> MVPSSPAVEKQVPVEPGPDPELRSWRHLVCYLCFYGFMAQIRPGESFITPYLLGPDKNFTREQVTNEITPVLSYSYLAVLVPVFLLTDYLRYTPVLLLQGLSFVSVWLLLLLGHSVAHMQLMELFYSVTMAARIAYSSYIFSLVRPARYQRVAGYSRAAVLLGVFTSSVLGQLLVTVGRVSFSTLNYISLAFLTFSVVLALFLKRPKRSLFFNRDDRGRCETSASELERMNPGPGGKLGHALRVACGDSVLARMLRELGDSLRRPQLRLWSLWWVFNSAGYYLVVYYVHILWNEVDPTTNSARVYNGAADAASTLLGAITSFAAGFVKIRWARWSKLLIAGVTATQAGLVFLLAHTRHPSSIWLCYAAFVLFRGSYQFLVPIATFQIASSLSKELCALVFGVNTFFATIVKTIITFIVSDVRGLG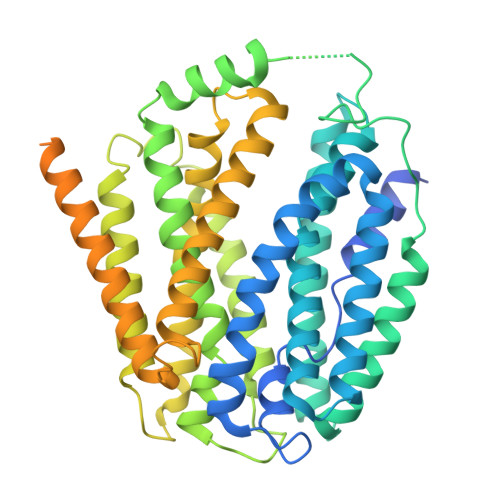LPVRKQFQLYSVYFLILSIIYFLGAMLDGLRHCQRGHHPRQPPAQGLRSAAEEKAAQALSVQDKGLGGLQPAQSPPLSPEDSLGAVGPASLEQRQSDPYLAQAPAPQAAEFLSPVTTPSPCTLCSAQASGPEAADETCPQLAVHPPGVSKLGLQCLPSDGVQNVNQ> QYSSNTQQGRTSIVHLFEWRWVDIALECERYLAPKGFGGVQVSPPNENVAIHNPFRPLWERYQPVSYKLCTRSGNEDEFRNMVTRCNNVGVRIYVDAVINHMCGNAVSAGTSSTCGSYFNPGSRDFPAVPYSGWDFNDGKCKTGSGDIENYNDATQVRDCRLSGLLDLALGKDYVRSKIAEYMNHLIDIGVAGFRIDASKHMWPGDIKAILDKLHNLNSNWFPEGSKPFIYQEVIDLGGEPIKSSDYFGNGRVTEFKYGAKLGTVIRKWNGEKMSYLKNWGEGWGFMPSDRALVFVDNHDNQRGHGAGGASILTFWDARLYKMAVGFMLAHPYGFTRVMSSYRWPRY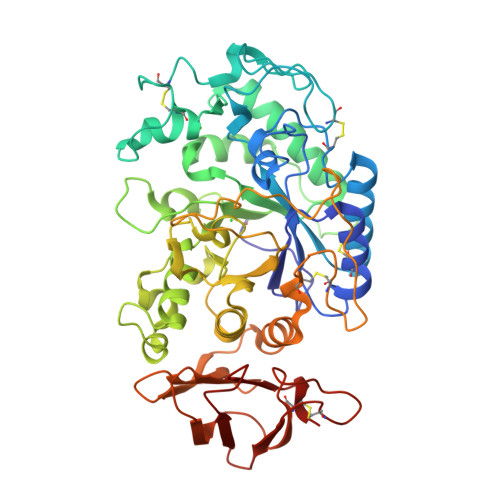FENGKDVNDWVGPPNDNGVTKEVTINPDTTCGNDWVCEHRWRQIRNMVNFRNVVDGQPFTNWYDNGSNQVAFGRGNRGFIVFNNDDWTFSLTLQTGLPAGTYCDVISGDKINGNCTGIKIYVSDDGKAHFSISNSAEDPFIAIHAESKL> KKAQPISVTMVTPAD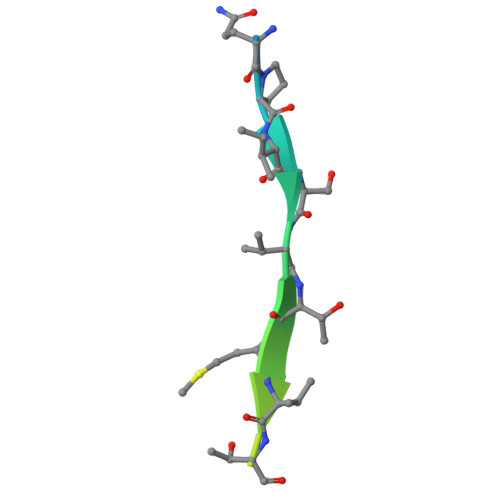LEPPQAKK Here we studied metal-preference evolution within the natural diversity of the iron/manganese superoxide dismutase (SodFM) family of reactive oxygen species scavengers. Only a few metalloenzymes have been rigorously demonstrated to be cambialistic in vivo, including some iron (Fe)- or manganese (Mn)-dependent superoxide dismutases (SODs; SodFMs); metalloenzymes that play an important role in cellular reactive oxygen species defence. To study this process, we leveraged the existence of naturally Fe-specific, Mn-specific and flexible Fe/Mn-cambialistic SodFM homologues, which differentially utilize these metals to catalyse the detoxification of superoxide. By combining phylogenetics, biochemistry and structural biology, we demonstrate that SodFM metal utilization can be evolutionarily fine tuned by sliding along a scale between perfect manganese and iron specificities.

In the cambialistic SodFM2 from B. fragilis (b), all mutants displayed lower activity with Mn and the majority had higher activity with Fe, representing change towards its most likely ancestral Fe-preferring phenotype. c, For Fe-preferring CPR Wolfebacteria SodFM1 (CPR-His), mutations in both the XD-2 and water-coordinating H/Q residues were necessary to shift towards the inferred ancestral higher Mn activity. The likely ancestral phenotype was proxied by the closely related SodFM1 from more basal Wolfebacteria. g,h, Single mutants, but not double mutants, shifted metal preference of N. alba SodFM3 (g, Q/H mutant) and Woesearchaeota SodFM4 (h, VD-2A). d–f, Crystal structures of S. aureus SodFM1 LD-2G (d), B. fragilis SodFM2 GD-2T (e) and CPR-His SodFM1 VD-2G H/Q double mutant (f) were analyzed to investigate structural effects of these mutations. The structures in e and f were solved in this study. In some, such as CPR SodFM1 H/Q VD-2G, only a cumulative effect of the two mutations affected the metal-preference, whereas no significant effect was observed in either single or double mutants of nanoarchaeon Nanopusillus acidilobi SodFM4. To further test the wider evolutionary significance of the secondary coordination sphere residues, we investigated double mutant variants combining mutations at positions XD-2 and the water-coordinating Q/HCterm. Our characterization of these variants revealed multiple evolutionary pathways towards metal-preference switching. Importantly, consistent with previous reports, comparison of four protein crystal structures of the WT and mutant SodFMs we determined here indicated that metal-preference modulation by XD-2 and Q/H occurs without any significant changes to the secondary metal coordination sphere within the resolution limits of the solved structures. This provides further support for ‘redox tuning’ via subtle structural changes.

>[2x]MKHELPPLPYAYNALEPFIDAKTLEIHHTKHHQSYVDKLNAALEKYPDLQDKTVEELIKSLNELPEEIRTTVRNNAGGHFSHTLYWNIMNPATQEYIPEELGNALVETFGSIIAFKEQFSKAAANIFGSGWVWLAADANKKLKIVSTTGQDNPLMTGDAPLMGIDIWEHAYYLHYQNRRPEYIENWWNVLDWKAVEERYNALG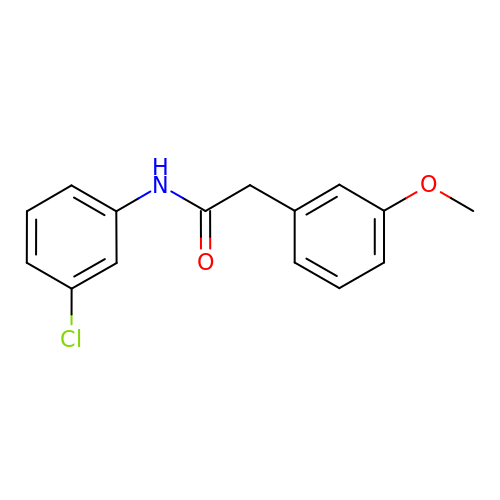N-(3-chlorophenyl)-2-(3-methoxyphenyl)acetamide | C15 H14 Cl N O2 | NQDLKNWLTCKGFR-UHFFFAOYSA-N> LAVIPILVIACDRSTVRRCLDKLLHYRPSAELFPIIVSQDCGHEETAQVIASYGSAVTHIRQPDLSNIAVQPDHRKFQGYYKIARHYRWALGQIFHNFNYPAAVVVEDDLEVAPDFFEYFQATYPLLKADPSLWCVSAWNDNGKEQMVDSSKPELLYRTDFFPGLGWLLLAELWAELEPKWPKAFWDDWMRRPEQRKGRACVRPEISRTMTFGRKGVSHGQFFDQHLKFIKLNQQFVPFTQLDLSYLQQEAYDRDFLARVYGAPQLQVEKVRTNDRKELGEVRVQYTGRDSFKAFAKALGVMDDLKSGVPRAGYRGIVTFLFRGRRVHL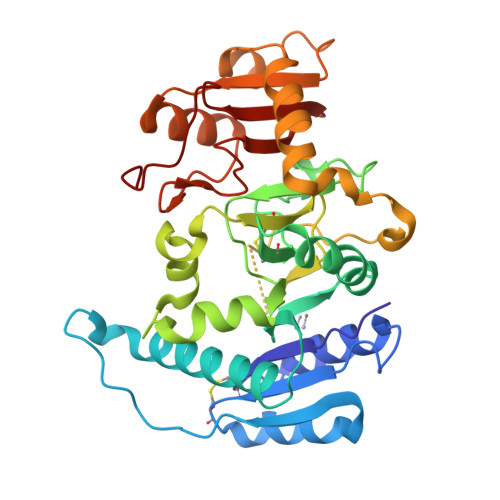APPQTWDGYDPSWT>MPPHGELQYLGQIQHILRCGVRKDDRTGTGTLSVFGMQARYSLRDEFPLLTTKRVFWKGVLEELLWFIKGSTNAKELSSKGVKIWDANGSRDFLDSLGFSTREEGD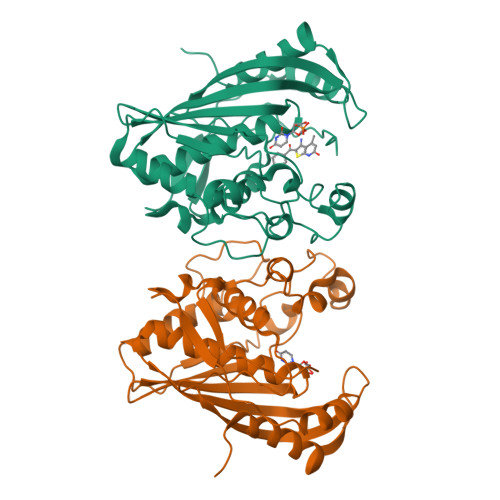LGPVYGFQWRHFGAEYRDMESDYSGQGVDQLQRVIDTIKTNPDDRRIIMCAWNPRDLPLMALPPCHALCQFYVVNSELSCQLYQRSGDMGLGVPFNIASYALLTYMIAHITGLKPGDFIHTLGDAHIYLNHIEPLKIQLQREPRPFPKLRILRKVEKIDDFKAEDFQIEGYNPHPTIKMEMAV[6x]> MGPQDNSLVIGASQEPRVLAGDFLRVISNQAIKSEIEQYLFAPFIGFNADSQNFPVLATEVPTLENGRLRVTDIGGGKKRLEMDITIRPDAKWSDGRPITTEDVAFYFEVGKAKGMPVLNPDFWERVNVRIKDARNFTLIFEPAYYYDTYGPINTYAPKHIMGPEWERVKAAARGLDPDKDAEKLNELYRNFFLKFATPQALNRGAMVYSGPFKLKRWVPGNSIEMERNPNFPIKPEGGESKYVQKVVY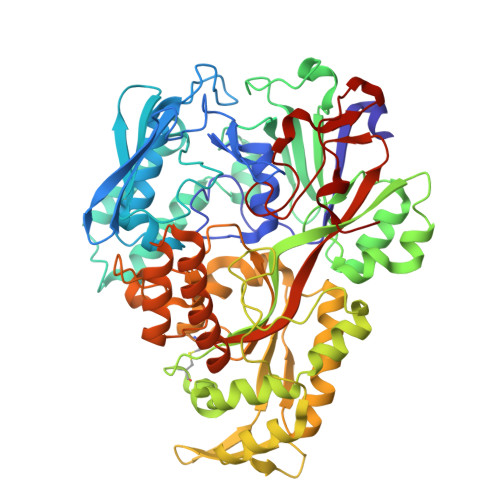RFIQNTNSLLVAVIGGSIDATSSVSLTFDQGRSPQLVRRAPGRFDIWFVPGAIWEHIDINKFENCQVVKDLGLNDKRTRQAILHALNREGLVKAFFDGLQPVAHTWIAPVNPLFNPNVKKYEFDLKKAEALLAEMGWRKGPDGILQRTVNGRTVRFEIEYVTTAGNVVRERTQQFFAEDLKKIGIAVKINNAPSAVVFADEFIQRASECKWTGMFEFAWVSNLQEDGSLFQYKNLNTGAIMVPTKENNYQGQNIGGWRNDEFDRLTSQAVLEFDPERRKQLFWRAQEIWAEELPALPLYFRANPYVVRKGLVNYVASAYSGGYGYPGWNAWEIGWESRGAVKKWDQAKYALSTR>[3x]MLDGAEASNGVSKQTVGGVHVTPEMLESVQIPLEADKVGMTPAEKSKLVNAATAVYIDMAVEEMRSRGLAPKADYRVHWWKVMQDFVDSGEGQRVLQETSLTNQELERVIAKLGIEGEVIARMGPEIVNILTGKTHALAHIMRDDLLFRVYLSDEGRRANRYMAEYARLLTSQRRDIRILEIGAGTGGTTSEVLNLCSPNGESFCAEYM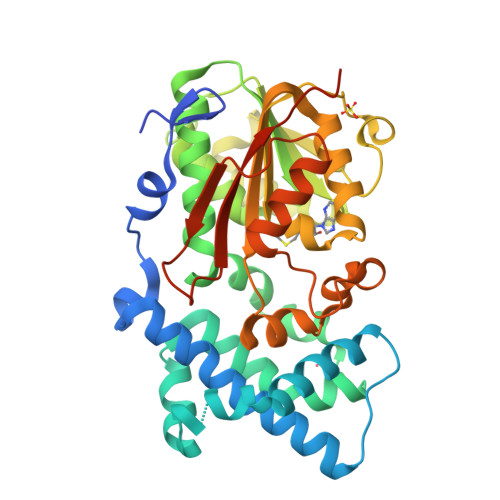YTDLSPGFFNAAKTTLKKWESHLAFQVLNIEDDPAGQGFKEHTYDLIIAANVIHATARLTNTLSNVHKLLKPGGVFGLVELTRLTPFYNLTFGSLSGWWAGVDEGRTESPLQSPQQWNSLLKQTGFSGVDLAAYDLPGPERHSCLLLSTALSNSVTTNGHGHHHHHHHH> MILRTSEETISTVQEKQQNISPLVRERGPQRVAAHITGTRGRSNTLSSPNSKNEKALGRKINSWESSRSGHSFLSNLHLRNGELVIHEKGFYYIYSQTYFRFQEEIKENTKNDKQMVQYIYK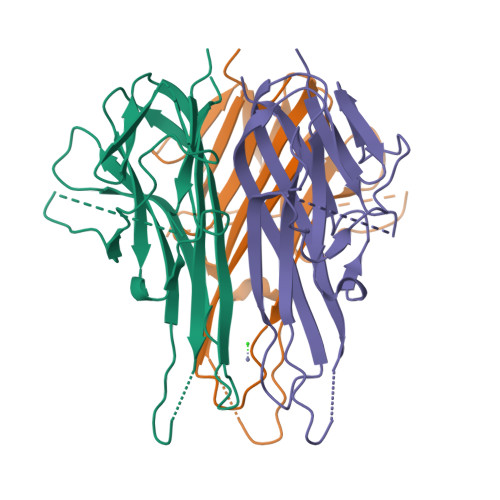YTSYPAPILLMKSARNSCWSKDAEYGLYSIYQGGIFELKENDRIFVSVTNEHLIDMDHEASFFGAFLVG>MGHHHHHHHHHHSSGHIEGRHMSRFAADPHWLIYLPPTMSPCETSKKEGMLEHPIEAFEYFRTRGVGKVVCEQKHMGSRAVVIVCKDSQVAEKRFGVLDGTAGICYTRTGRHFFDDMQLEAELIDRVRKVLDKSGFWGDFNTDWVCLDCELMPWSAKAQKLLEEQYSAVGISGRVVLDEAVKLLKQASLNKTVSFDVSRQTSGKNADINELLQRFTERSEMMQKYVEAYRKYCWPVNSIDDLKLAPFHILATEGKVHSDKNHIWHMDTIAKYCTQDDSLIMATNHILVDVTDAESVDKGIKWWEDLTASGGEGMVVKPYDFIVKNGRELLQPAVKCRGREYLRIIYGPEYTMDENIER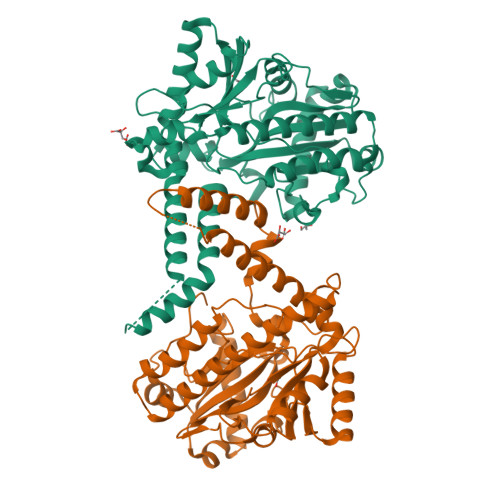LRNRAVGKKRSLALREFSLGMEALERFVRNEPLYRVHECVFGVLALESEPVDPRL[2x]4-[(~{Z})-1-cyano-2-[6-[2-hydroxyethyl(methyl)amino]pyridin-3-yl]ethenyl]benzenecarbonitrile | C18 H16 N4 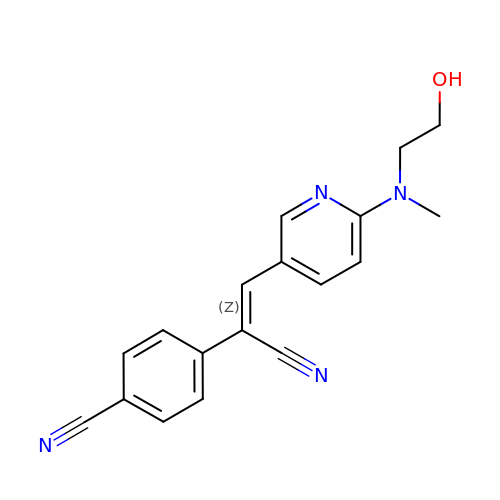O | MMFJPNCXBGQMOQ-LICLKQGHSA-N>MSSSGIVLYGTDLSPCVRTVKLTLKVLNLDYEYKEVNLQAGEHLSEEYVKKNPQHTVPMLDDNGTFIWDSHAIAAYLVDKYAKSDELYPKDLAKRAIVNQRLFFDASVIYASIANVSRPFWINGVTEVPQEKLDAVHQGLKLLETFLGNSPYLAGDSLTLADLSTGPTVSAVPAAVDIDPATYPKVTAWLDRLNKLPYYKEINEAPAQSYVAFLRSKWTKLGDK[2x]

Glutathione transferases (GSTs) are enzymes found universally across all kingdoms of life, spanning more than six decades of research. In insects, they play pivotal roles in various processes, including detoxification, ecdysteroid biosynthesis, or chemoperception. GSTs were categorized into four types based on the catalytic amino acids, namely, tyrosine (TyrGSTs), serine (SerGSTs) including the Delta and Epsilon classes, cysteine (CysGSTs), and atypical (AtyGSTs). All the GSTs’ classes identified within the insects are recognized as dimeric including the Delta and Epsilon.

The crystal structure of DmGSTE1 was solved at 1.80 Å resolution in the P212121 space group. The asymmetric unit contains one dimer of DmGSTE1. Each subunit adopts the typical GST fold with an N-terminal thioredoxin domain (β1α1β2α2β3β4α3, Ser2-Tyr88) and an all-helical C-terminal domain (α4α5α6α7α8, Pro89-Asp223). The glutathione binding site (G site) is occupied by a mixture of glutathione and glutathione sulfoxide refined with equal occupancies. The sulfur atom of the reduced form of glutathione is oriented towards the solvent, while the sulfoxide group of the oxidized form establishes a hydrogen bond with the Ser14 sidechain. This Ser14 is part of the catalytic motif ‘SPCV’ at the N-terminal end of helix α1 of DmGSTE1. Interestingly, the Cys16 residue part of this same catalytic motif is oriented toward the solvent and could be responsible for the thiol transferase activity observed with HED, as observed previously for other Ser-GSTs harboring a Cys in the catalytic motif. The clasp residue around the axis of the dimer was Phe103, as predicted from the sequence alignment. Both Phe103A and Phe103B interacted by Π-Π stacking, similar to GST Delta, while most GST Epsilon structures had a His. In summary, the overall assembly was stabilized by a combination of polar interactions surrounding the hydrophobic core of the dimer with the clasp Phe103 as a central and crucial anchor point.>ATTYNAVVSKSSSDGKTFKTIADAIASAPAGSTPFVILIKNGVYNERLTITRNNLHLKGESRNGAVIAAATAAGTLKSDGSKWGTAGSSTITISAKDFSAQSLTIRNDFDFPANQAKSDSDSSKIKDTQAVALYVTKSGDRAYFKDVSLVGYQDTLYVSGGRSFFSDCRISGTVDFIFGDGTALFNNCDLVSRYRADVKSGNVSGYLTAPSTNINQKYGLVITNSRVIRESDSVPAKSYGLGRPWHPTTTFSDGRYADPNA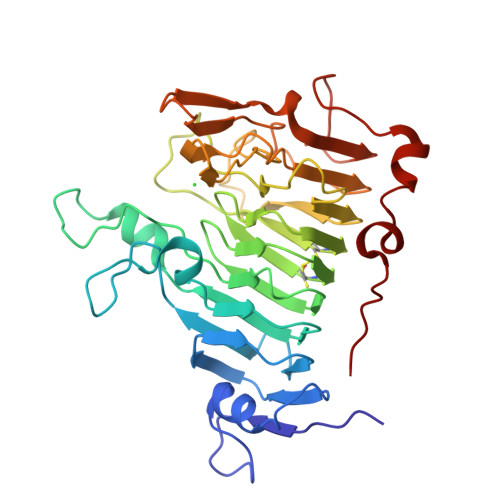IGQTVFLNTSMDNHIYGWDKMSGKDKNGNTIWFNPEDSRFFEYKSYGAGAAVSKDRRQLTDAQAAEYTQSKVLGDWTPTLP[2x]> MPKALRFLGWPVLVGVLLALLIIQHNPELVGLPRQEVHVEQAPLLSRLQEGPVSYANAVSRAAPAVANLYTTKMVSKPSHPLFDDPMFRRFFGDNLPQQKRMESSLGSAVIMSAEGYLLTNNHVTAGADQIIVALRDGRETIAQLVGSDPETDLAVLKIDLKNLPAMTLGRSDGIRTGDVCLAIGNPFGVGQTVTMGIISA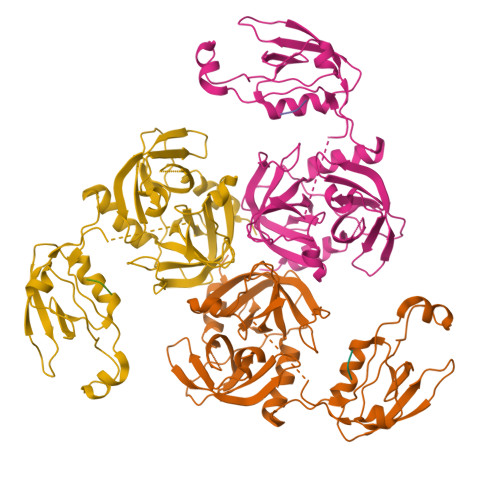TGRNQLGLNTYEDFIQTDAAINPGNAGGALVDAAGNLIGINTAIFSKSGGSQGIGFAIPTKLALEVMQSIIEHGQVIRGWLGVEVKALTPELAESLGLGETAGIVVAGVYRDGPAARGGLLPGDVILTIDKQEASDGRRSMNQVARTRPGQKISIVVLRNGQKVNLTAEVGLRPPPAPAPQQKQDGGE;> WVF> GPLGSPYTIELIQPEDGEAVIAMLKTFFFKDEPLNTFLDLGECKELEKYSLKPLPDNCSYKAVNKKGEIIGVFLNGLMRRPSPDDVPEKAADSCEHPKFKKILSLMDHVEEQFNIFDVYPDEELILDGKILSVDTNYRGLGIAGRLTERAYEYMRENGINVYHVLCSSHYSARVMEKLGFHEVFRMQFADYKPQGEVVFKPAAPHVGIQVMAKEV

Acetyl coenzyme A (Ac-CoA)-dependent N-acetylation is performed by arylalkylamine N-acetyltransferase (AANAT) and is important in many biofunctions. Dopamine N-acetyltransferase (Dat) is the first identified insect AANAT from Drosophila melanogaster. Dat exhibits an ordered sequential mechanism in which the cofactor (Ac-CoA) binds first, followed by the binding and acetyl transfer of the substrate. Overall structures revealed that Dat was a globular protein containing a tunnel-like cavity, a substrate located in the middle of the protein, a CoA group located at the bottom, and an acetyl group between the substrate and CoA.

To distinguish the roles of the acetyl group and the CoA moiety in the regulation of conformational changes, the crystal structure of the Dat/CoA complex was solved at a resolution of 1.45 Å as a control to compare with the Dat/Ac-CoA complex. In the Dat/CoA complex, there was no additional α9, and the position of α7 was different, indicating that the formation of α9 and the shift of α7 occurred in the presence of the acetyl group. Because the interactions between α9 and the shifted α7 were critical for catalytic site, this result also supported that the acetyl group fine-tuned the catalytic site through forming α9 to interact with α7. In contrast, the locations of α5 and the critical salt-bridge interactions of Asp46–Arg153 and Lys192–CoA moiety were very similar in these two binary complexes, indicating that the conformational changes for stabilizing bound cofactor were regulated by the CoA moiety. Because the Asp46–Arg153 salt bridge was also observed in the Dat/CoA complex, we further concluded that the structural switch sensed the occupancy of the CoA moiety at the cofactor-binding site, which is different from the suggestion of Aboalroub et al. (sensing the acetyl group). The replacement of the bound CoA by Ac-CoA is possible because the Kd of Ac-CoA binding to Dat (5.51 ± 1.92 μM) is ~30-fold lower than that of CoA (152.89 ± 26.48 μM). However, in the case of Dat, differential scanning calorimetry (DSC) data revealed that the thermal stability of Dat/CoA was higher than that of apo-Dat and lower than that of Dat/CoA/Ac-PEA, while Tm of Dat/Ac-CoA and Dat/CoA/Ac-PEA were almost the same.> QTQPVPRFDETSTDTGGP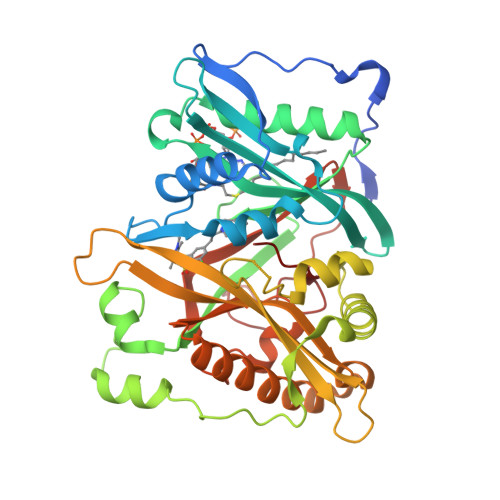IKIIDPEKVSKEPDALLEGFEWATLDLTNETELQELWDLLTYHYVEDDNAMFRFRYSQSFLHWALMSPGWKKEWHVGVRATKSRKLVASICGVPTEINVRNQKLKVVEINFLCIHKKLRSKRLTPVLIKEITRRCYLNGIYQAIYTAGVVLPTPVSSCRYYHRPLDWLKLYEVGFSPLPAGSTKARQITKNHLPSTTSTPGLRPMEPKDIDTVHDLLQRYLSRFALNQAFTREEVDHWLVHKPETVKEQVVWAYVVEDPETHKITDFFSFYNLESTVIQNPKHDNVRAAYLYYYATETAFTNNMKALKERLLMLMNDALILAKKAHFDVFNALTLHDNPLFLEQLKFGAGDGQLHFYLYNYRTAPVPGGVNEKNLPDEKRMGGVGIVML>[2x]MHISDEQLKRPLRDYGEALEMWSTFQTKTQALSQSLSSQLRLILTGSGIPSKRAYQILLCVDDSSSMSDDNRSTAGNLALESLVMVARALTVLEAGQIGVMGFGTDVFVAHALTDPPFTSQDAGARVLQQFTFRQDSTDMVLLLRRTIDHFREARLIQASSSRGGEDLWQLALILSDGLVQSRDHA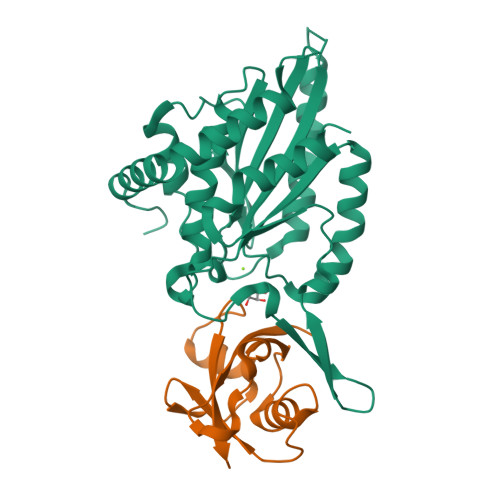RLRPLLREAMEQRVMVVFIVMDDARSRKGHSVLELKEARFGPDGVPVIHRYLDSFPFPYYLIVHHLEDLPGALAALLRTWFAEVNSGSHHHHHH;>[2x]MKHHHHHHPMAPAPVAQVKVIFTTTEPDLELPESKRQLLVPADIRRYGLSRILNSESMLDTGSIPFDFLINGSFLRSSLEDYLTSNGLSLETTLTLQYVRS>SKEIDISCVKIEQVIGAGEFGEVCSGHLKLPGKREIFVAIKTLKSGYTEKQRRDFLSEA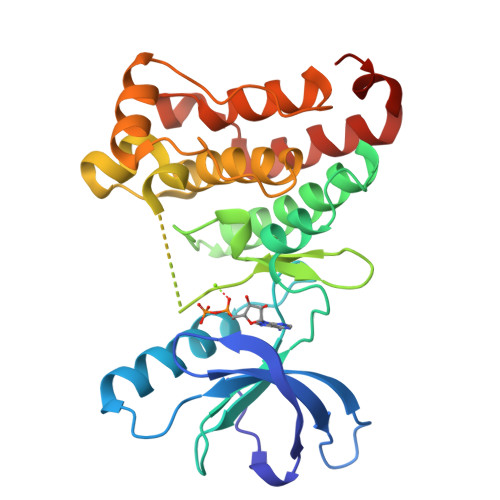SIMGQFDHPNVIHLEGVVTKSTPVMIITEFMENGSLDSFLRQNDGQFTVIQLVGMLRGIAAGMKYLADMNYVHRALAARNILVNSNLVCKVSDFGLSRFLEDDTSDPTYTSALGGKIPIRWTAPEAIQYRKFTSASDVWSYGIVMWEVMSYGERPYWDMTNQDVINAIEQDYRLPPPMDCPSALHQLMLDCWQKDRNHRPKFGQIVNTLDKMIRNPNSLKAMAPLSS[4x]>MAAYTDVPISGMRKTIAARLKESVTENPHFFVSTNLSVSKLLKLRQALNSSADGRYKLSVNDFLIKAMGIASKRVPTVNSSWRDGVIRQFETVDVSVAVATPNGLITPIVKGVEGKGLESISAAVKELAKKARDGKLKPEEYQGGSISISNMGMNPAVQSFTAIINPPQAAILAVGAPQKVAVPVENEDGTTGVSWDEQIIVTASFDHKVVDGAVGAEWIRELKKVIENPLELLL[6x];>HHHHHHSQDPNSSPSSENLYFQSPAPPPVAVVTAPISLSAAIDVQNKLHKTIGVFLPLSTFITRATEIANQKLPLPANYQPTADELFNQVLGLDKVTRKESRGSYTPTFGSFVAPQRAARKADIIDILAAPSTRVAASAQSKSAAPGLTTSGPNVFS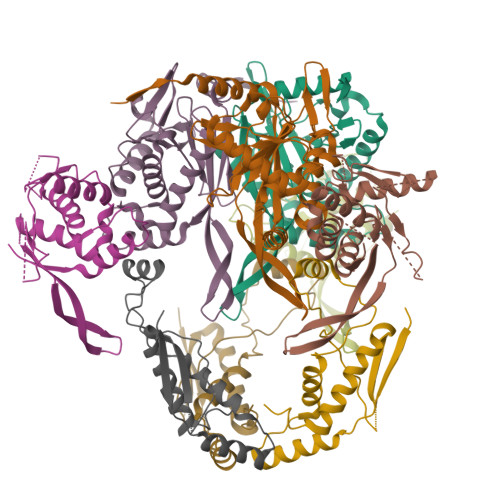LQVPKSEEKRAQAFLQKMKLVLEQEPDKLVRA[3x]> GPGSDDEINAQSVWSEEISSNYPLCIKNLMEGLKKNHHLRYYGRQQLSLFLKGIGLSADEALKFWSEAFTRNGNMTMEKFNKEYRYSFRHNYGLEGNRINYKPWDCHTILSKPRPGRGDYHGCPFRDWSHERLSAELRSMKLTQAQIISVLDSCQKGEYTIACTKVFEMTHNSASADLEIGEQTHIAHPN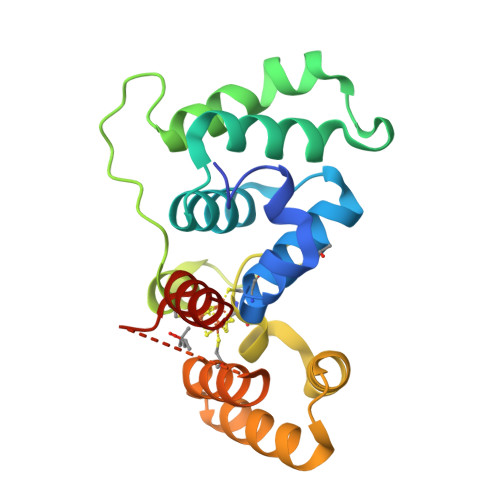LYFERSRQLQK>[2x]MAQLTTESMPFNVAEGKEVLLLVHNLPQQLFGYSWYKGERVD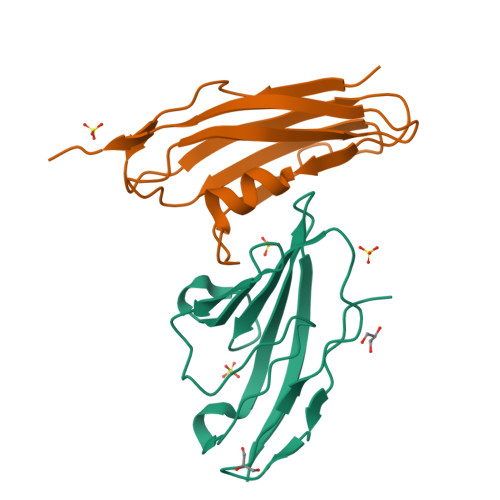GNRQIVGYAIGTQQATPGPANSGRETIYPNASLLIQNVTQNDTGFYTLQVIKSDLVNEEATGQFHVY;>[2x]ANENNQQKIELTVSPENITVYEGEDVKFTVTAKSDSKTTLDFSDLLTKYNPSVSDRISTNYKTNTDNHKIAEITIKNLKLNESQTVTLKAKDDSGNVVEKTFTITVQKKEEKQLPSTGGSHHHHHH>HHHHHHSSGLVPRGSHMMGVEEHKKEAPKTFKFGVITVSDKGAKGEREDKSGPLIIEELSKLGEHVYYKIVPDDKIEVLIALFEAIKSGADVVVTTGGTGITRRDITIESIKPLFDKELSFGEVFRAKSYEEVGYATVLTRATAGIIRGQERIVVVFSLPGSVNAVKTGLEIIKSEV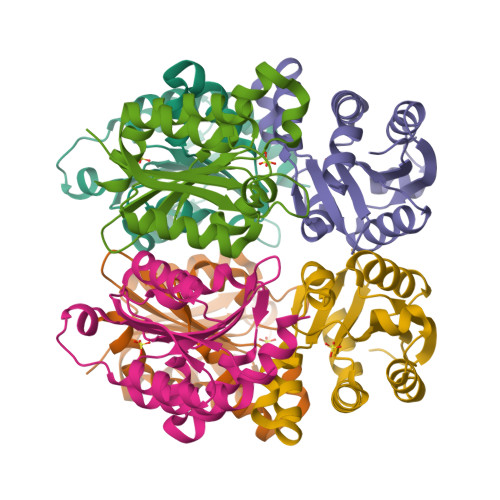FHILKHARE[3x]>GAMALPSGSDPAFSQPKSVLDAGLTCQGASPSSVSKPILLVPGTGTTGPQSFDSNWIPLSAQLGYTPCWISPPPFMLNDTQVNTEYMVNAITTLYAGSGNNKLPVLTWSQGGLVAQWGLTFFPSIRSKVDRLMAFAPDYKGTVLAGPLDALAVSAPSVWQQTTGSALTTALRNAGGLTQIVPTTNLYSATDEICQPQVSNSPLDSSYLFNGKNVQAQAVCGPLFVIDHAGSLTSQFSYVVGRSALRSTTGQARSADYGITDCNPLPANDLTPEQKVAAAALLAPGVAAIVAGPKQNCEPDLMPYARPFAVGKRTCS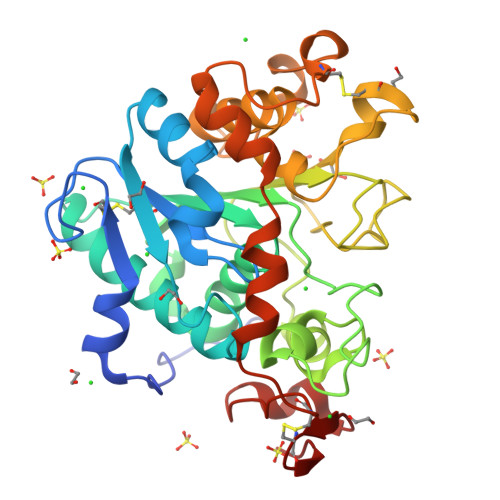GIVTP[2x]> MSKAKIGIVTVSDRASAGITADISGKAIILALNLYLTSEWEPIYQ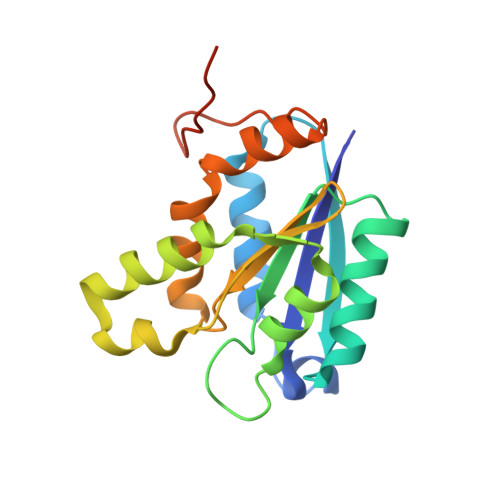VIPDEQKVIERTLIKMADIQDCCLIVTTGGTGPAKRDVTPEATEAVCDRMMPGFGELMRAESLKEVPTAILSRQTAGLRGDSLIVNLPGDPASISDCLLAVFPAIPYCIDLMEGPYLECNEAMIKPFRPKAKLEHHHHHH> MELAEKDKGRDFTLRNARMDDIDQIIKINRLTLPENYPYYFFVEHLKEYGLAFFVAIVDNSVVGYIMPRIEWGFSNIKQLPSLVRKGHVVSIAVLEEYR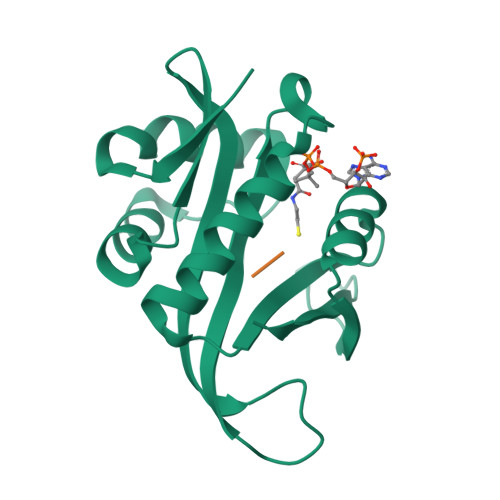RKGIATTLLEASMKSMKNDYNAEEIYLEVRVSNYPAIALYEKLNFKKVKVLKGYYADGEDAYLMARPLHHHHHH;> SSGTPT(2R)-2-aminoheptanedioic acid | 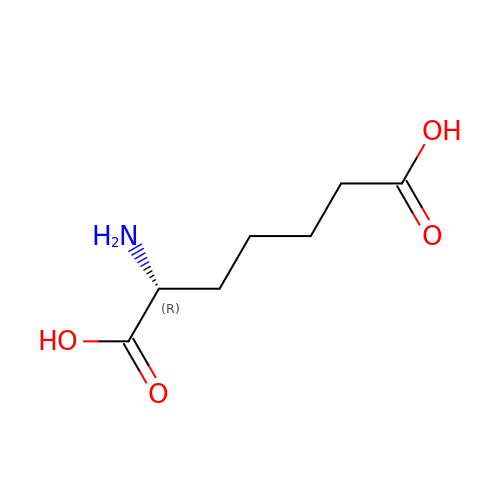C7 H13 N O4 | JUQLUIFNNFIIKC-RXMQYKEDSA-N> MPQSKSRKIAILGYRSVGKSSLTIQFVEGQFVDSYDPTIENTFTKLITVNGQEYHLQLVDTAGQDEYSIFPQTYSIDINGYILVYSV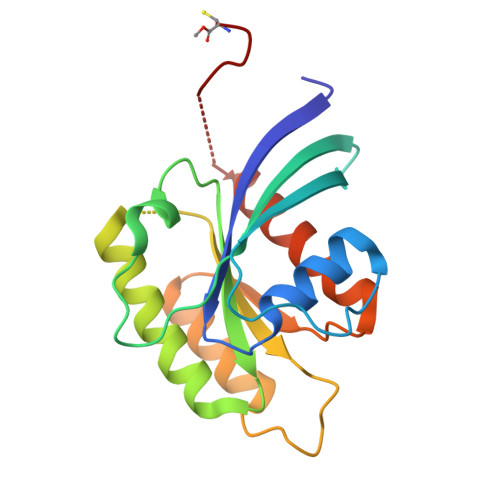TSIKSFEVIKVIHGKLLDMVGKVQIPIMLVGNKKDLHMERVISYEEGKALAESWNAAFLESSAKENQTAVDVFRRIILEAEKMDGACSQGKSSC3-DEHYDROSHIKIMATE | C7 H10 O5 | 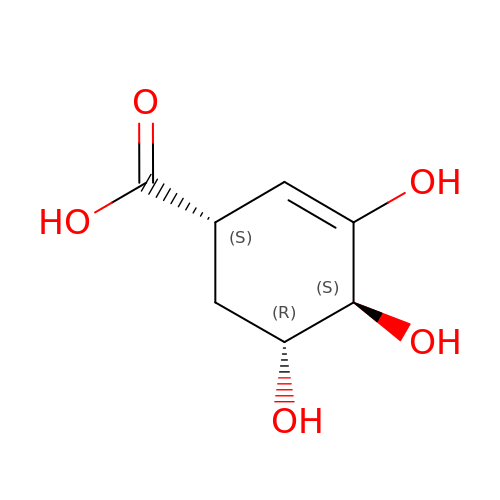YVYKOQWMJZXRRM-UYFOZJQFSA-N>GELETKAVGMSNDGRFLKFDIEIGRGSFKTVYKGLDTETTVEVAWCELQDRKLTKSERQRFKEEAEMLKGLQHPNIVRFYDSWESTVKGKKCIVLVTELMTSGTLKTYLKRFKVMKIKVLRSWCRQILKGLQFLHTRTPPIIHRDLKCDNIFITGPTGSVKIGDLGLATLKRADFAKSVIGTPEFMAPEMYAAAYDESVDVYAFGMCMLEMA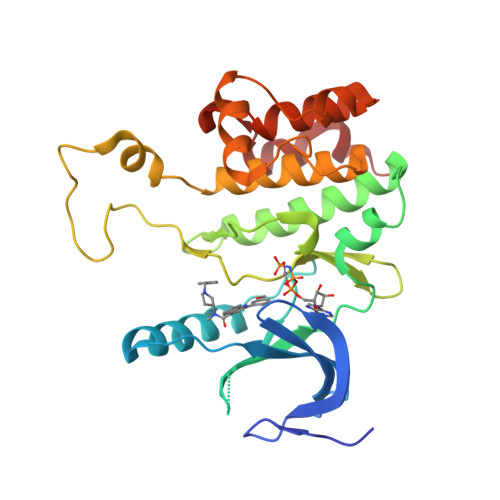TSEYPYSECQNAAQIYRRVTSGVKPASFDKVAIPEVKEIIEGCIRQNKDERYSIKDLLNHAFFQEET[2x]> AAAAAAAAAAA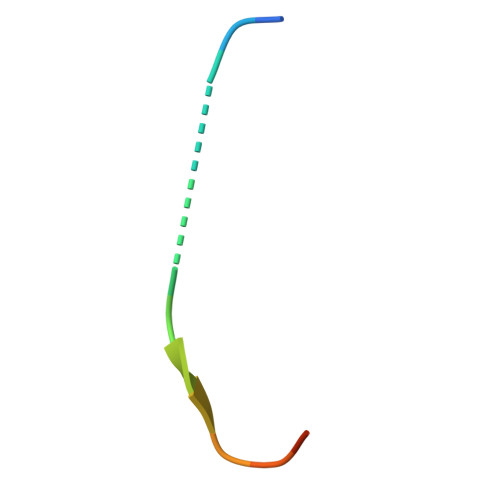A> MPKLPRG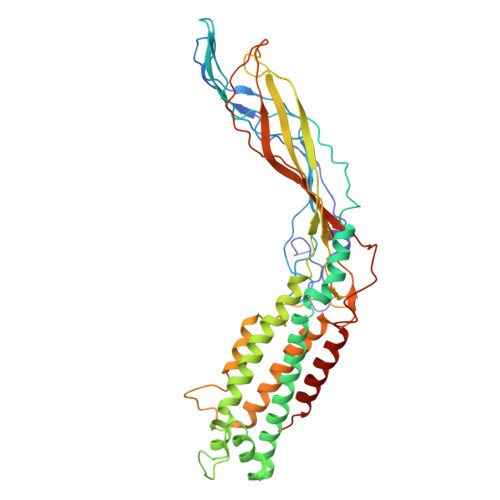LRFGADNEILNDFQELWFPDLFIESSDTHPWYTLKGRVLNAHLDDRLPNVGGRQVRRTPHRVTVPIASSGLRPVTTVQYDPAALSFLLNARVDWDFGNGDSANLVINDFLFRTFAPKEFDFSNSLVPRYTQAFSAFNAKYGTMIGEGLETIKYLGLLLRRLREGYRAVKRGDLRALRRVIQSYHNGKWKPATAGNLWLEFRYGLMPLFYDIRDVMLDWQNRHDKIQRLLRFSVGHGEDYVVEFDNLYPAVAYFKLKGEITLERRHRHGISYANREGYAVFDNGSLRPVSDWKELATAFINPHEVAWELTPYSFVVDWFLNVGDILAQQGQLYHNIDIVDGFDRRDIRLKSFTIKGERNGRPVNVSASLSAVDLFYSRLHTSNLPFATLDLDTTFSSFKHVLDSIFLLTQRVKR>MSSGGDPSEDTGAGDGEQGGESSAMAGRSGGGMGGGGGGGGSVGFSTGGWEGGTYFSDHTVTTTNTRQWYTGILNGHRYSKLAQTTGSNLQAAKPWVGIQTPWAYLNLNCYHCHFSPQDWQRLLNEYKAWRPKRMHVRIYNLQIKQITTVGADTLYQNDLTAGVHIFCDGSHQYPYAQHPWDEGASPELPNEIWKLPQYAYFQYQGDLTDHATANTPQNVESMLRSNIPLFLLENSNHEVLRTGEMTEFSFTFQSGWVTNDRAYCCPQSDFNPLVQTRRYYPTWNGSSNSYSYNRYGPYKKPSNWMPGP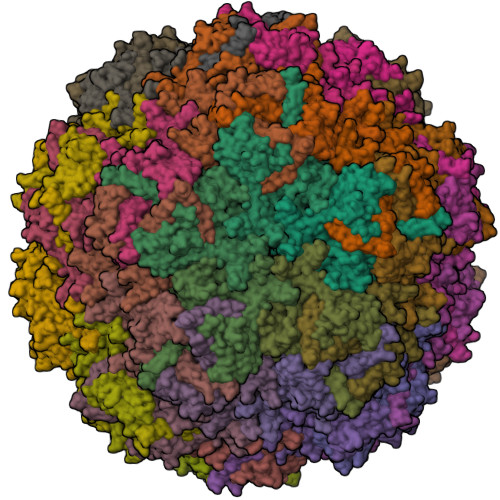GLAYKGATHTNQNPDDARGPIVTTIAPRGTISVGSTPSNDAPNDGDNTISSDGVKQGGWQTAPVNGACSRTDYPTLAFDPSDRSTNQNIPTRNLDIDMTRWYRVHEPVRSGNGSTYYNVDDVWMYPNQVWNSTPICRDNPIWDKVPRTDHHTLLDSSDGTLPMKHPPGNIFIKCAKIPIPTSNNTDSYLNIYVTGQVTYTVEWEVQRYQTKNWRPELRTSAGTYNQHEIYNIGENGTYNRANTFNECMPTKCGINRVL[60x]> MSLINEATLAESIRRLRQGERATLAQAMTLVESRHPRHQALSTQLLDAIMPYCGNTLRLGVTGTPGAGKSTFLEAFGMLLIREGLKVAVIAVDPSSPVTGGSILGDKTRMNDLARAEAAFIRPVPSSGHLGGASQRARELMLLCEAAGYDVVIVETVGVGQSETEVARMVDCFISLQIAGGGDDLQGIKKGLMEVADLIV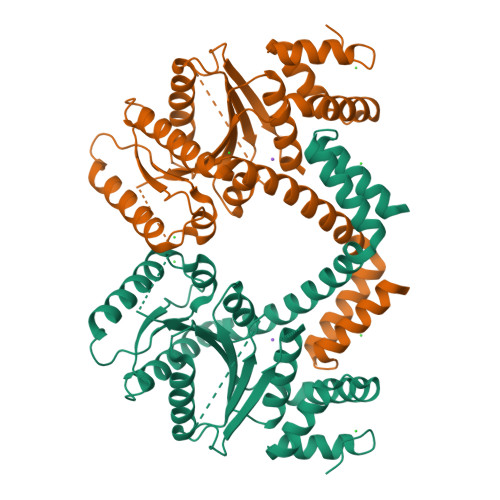INKDDGDNHTNVAIARHMYESALHILRRKYDEWQPRVLTCSALEKRGIDEIWHAIIDFKTALTASGRLQQVRQQQSVEWLRKQTEEEVLNHLFANEDFDRYYRQTLLAVKNNTLSPRTGLRQLSEFIQTQYFDEGHHHHHH> GSHMDAAPCVVNLSSSNLKFEIIPQELHARLLDQE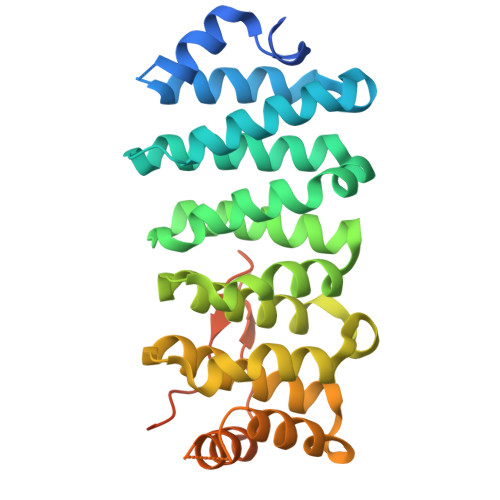DYKNRTQAVEELKQLLGKFNPSSTPHASLVGFISLLYNLLDDSNFKVVHGTLQVLHLLVIRLGEQVQQFLGPVIAASVKVLADNKLVIKQEYMKIFLKLMKEVGPQRVLSLLLENLKHKHSRVREEVVNICICSLLTYPSEDFDLPKLSFDLAPALVDSKRRVRQAALEAFAVLASSMGSGKTNVLFKAVDTVELQDNGDGVMNAVQARLARKTLPRLTEQGFVEYAILMPSSAQGRSSHLAHGADTDWLMSGNRTQS>[12x]MFERFTDRARRVVVLAQEEARMLNHNYIGTEHILLGLIHEGEGVAAKSLESLGISLEGVRSQVEEIIGQGQQAPSGHIPFTPRAKKVLELSLREALQLGHNYIGTEHILLGLIREGEGVAAQVLVKLGAELTRVRQQVIQLLSGYKLAAALEHHHHHH

ClpC1 is an ATP-dependent homohexamer that is responsible for substrate recognition and unfolding. ClpC1 is a 95 kDa caseinolytic AAA+ protein with an N-terminal domain (NTD) and two nucleotide-binding domains (D1 and D2). The essential ClpC1–ClpP1–ClpP2 proteasome complex of Mtb has recently become the focus of several drug-discovery campaigns. The NTD (amino acids 1–145) has been studied extensively to determine the most critical residues for the binding of ClpC1 to several natural cyclopeptides with potent anti-TB activity.

The structure of the potent antituberculosis macrocyclic depsipeptide ecumicin complexed with the N-terminal domain of ClpC1 (ClpC1-NTD) is presented here. Crystals of the ClpC1-NTD–ecumicin complex were monoclinic (unit-cell parameters a = 80.0, b = 130.0, c = 112.0 Å, β = 90.07°; space group P21; 12 complexes per asymmetric unit) and diffracted to 2.5 Å resolution. The new structure of the ecumicin complex showed a unique 1:2 (target:ligand) stoichiometry exploiting the intramolecular dyad in the α-helical fold of the target N-terminal domain. The result is particularly surprising as structurally related (although smaller) hepta­cyclopeptides such as CYMA and RUF-I bound with a 1:1 ratio of target to ligand while occupying the same binding region. In the structure of the complex the nonpolar sides of the ECU molecules face each other across the intramolecular pseudo-dyad, which provides an additional hydrophobic surface of approximately 240 Å2 (15% of the total) for the second ECU molecule to bind. In site 1, the polar side of ECU (including its three-residue tail) serves as a very effective ‘anchor and guide’ to induce a conformational change in the four N-terminal residues of ClpC1-NTD (Met1-Phe2-Glu3-Arg4) and form an extended chain that distinctively differs from the short 310-helix found in the ClpC1-NTD–RUF-I complex. Based on the quality of the electron density for the tail residues of ECU and the interacting residues in ClpC1-NTD, it is probable that ECU binds to site 1 with higher affinity than to site 2. In the ECU complex the N-terminus is extended and the peptide tail swings around it, making significant contacts. In the packing of the long and extended asymmetric unit, clusters of three dimers arrange themselves in a looser hexameric arrangement. In addition, the SPR data on the mutants and the multi-site binding of ECU to ClpC1-FL provided further strong evidence for the unusual stoichiometry of the ClpC1-NTD–ECU complex (1:2) in solution.> X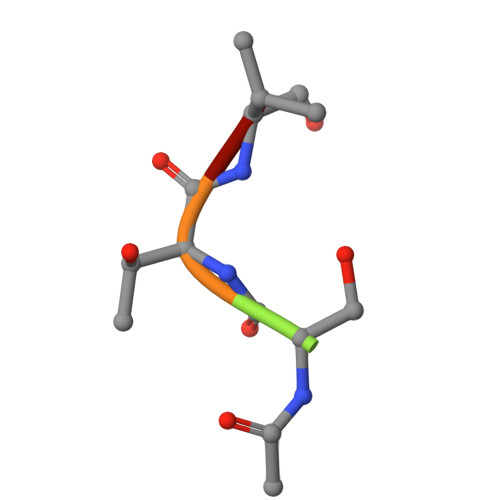STVG> LAAGTPALGDDRGRP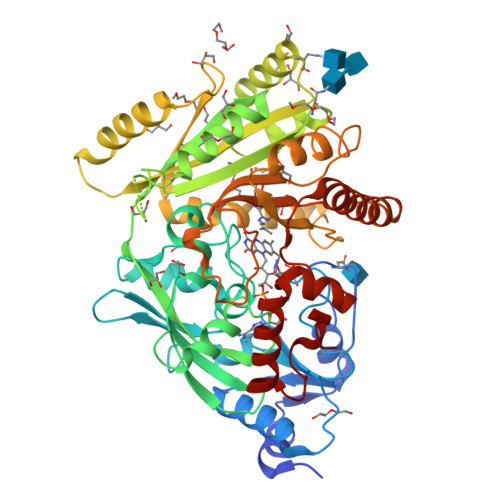WPASLAALALDGKLRTDSNATAAASTDFGNITSALPAAVLYPSSTADLVALLSAANSTPGWPYTIAFRGRGHSLMGQAFAPGGVVVNMASLGDAAAPPRINVSADGRYVDAGGEQVWIDVLRASLARGVAPRSWTDYLYLTVGGTLSNAGISGQAFRHGPQISNVLEMDVITGHGEMVTCSKQLNADLFDAVLGGLGQFGVITRARIAVEPAPARARWVRLVYTDFAAFSADQERLTAPRPGGGGASFGPMSYVEGSVFVNQSLATDLANTGFFTDADVARIVALAGERNATTVYSIEATLNYDNATAAAAAVDQELASVLGTLSYVEGFAFQRDVAYAAFLDRVHGEEVALNKLGLWRVPHPWLNMFVPRSRIADFDRGVFKGILQGTDIVGPLIVYPLNKSMWDDGMSAATPSEDVFYAVSLLFSSVAPNDLARLQEQNRRILRFCDLAGIQYKTYLARHTDRSDWVRHFGAAKWNRFVEMKNKYDPKRLLSPGQDIFN>[2x]MPR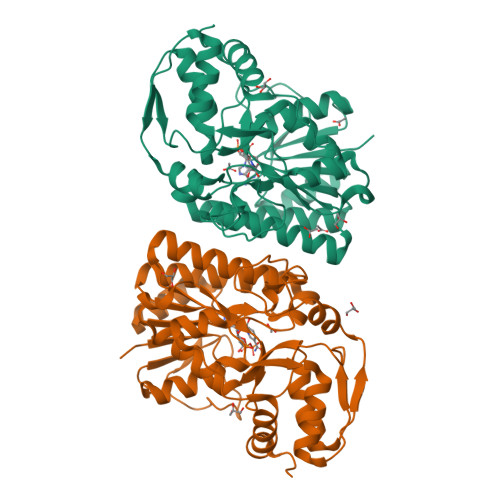VLVTGALGQIGTDLSLALRDKFGADSVLVSDVVEPGAKHPLAGLKGVEKLDCLDSNGFEKLVKEFKPTWMYHLPAIMSVRGEAEPDLAMDINVNTTRYALELARKYNIRIFIPSTIAAFGDKCGKTMTKDDTIMNPSTVYGVTKVYTELLGTWYRQKYGVDFRSVRLPGIISAATLPGGGATDYAIHMYHSALLQKKCVCPVLPYESLPMMYMPDTLNSLVKIMEAPLEKLTRTVYNITGFSFSPSELRFSIERCTDRTIEVEYVEGPAQKIANSWPDSLDDSNARNDWGHQVKYDIDMMSEDMLRQIPILHGLPSL A widely applicable approach is the use of photocaged substrates, where the photocage is soaked into the crystal in advance and then activated using a laser pulse to provide uniform initiation of the reaction throughout the crystal. This work characterizes photocage release of nitric oxide and binding of this ligand to two heme protein systems, cytochrome c′-β and dye-decolourizing peroxidase B using a fixed target sample delivery system. In this work, we describe a thorough characterization of the application of the NO photocage N,N′-bis-(carb­oxy­methyl)-N,N′-di­nitroso-1,4-phenyl­enedi­amine (henceforth referred to as NO cage) to room-temperature microcrystals of two proteins: a gas binding cytochrome c′ (McCP-β) and a dye-decolourizing peroxidase B (DtpB). Laser parameters for photoactivation are systematically explored, and time-resolved structures over timescales ranging from 100 µs to 1.4 s using synchrotron and XFEL beamlines are described. We have demonstrated a sample and time efficient approach using fixed targets to carry out time-resolved SSX and SFX experiments with an NO photocage over the microsecond to second time regimes.

Prior to utilizing the NO cage to characterize NO binding, we sought to obtain suitable control structures including both the ground state of the proteins (ligand free) and a ‘dark’ structure where the NO cage compound had been soaked into crystals but not activated by the laser pulse. McCP-β occurs within the methano­trophic Methyl­ococcus capsulatus (Bath) together with a homologous cytochrome P460 enzyme that oxidizes hydroxyl­amine with NO as a reaction intermediate. Possible roles for McCP-β include NO buffering to mediate toxicity/stress or transport between different enzymes that interact with NO. Firstly, upon NO binding, a vacant coordination position on the distal face of the heme iron becomes occupied, resulting in unambiguous electron density changes.

>[2x]ATKVKYPDGFRSWYHVKSMVIQPGHPLENPFGGIHHVYANAEAIQGLRGGNYPDGAVLVFDLFDYQEDNHALVEGKRKLIGVMERDAKRFSATGGWGYEGFGEGKPDKRLVTDGGQGCFGCHAAQKESQYVFSRLRD>[2x]TLQIQFKKYELPPLPYKIDALEPYISKDIIDVHYNGHHKGFVNGANSLLERLEKVVKGDLQTGQYDIQGIIRGLTFNINGHK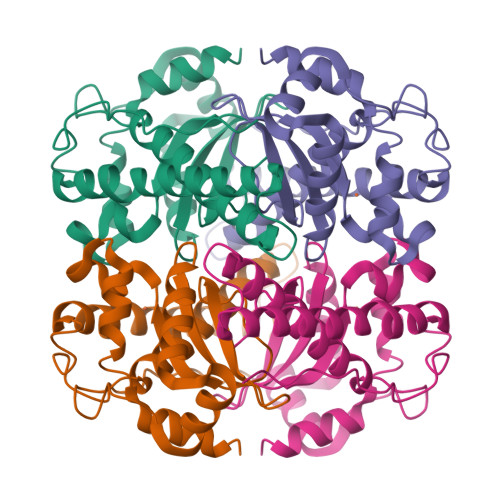LHALYWENMAPSGKGGGKPGGALADLINKQYGSFDRFKQVFTETANSLPGTGWAVLYYDTESGNLQIMTFENHFQNHIAEIPIILILDEFEHAYYLQYKNKRADYVNAWWNVVNWDAAEKKLQKYLTK>[2x]MEAPEFKDFAKTMVDF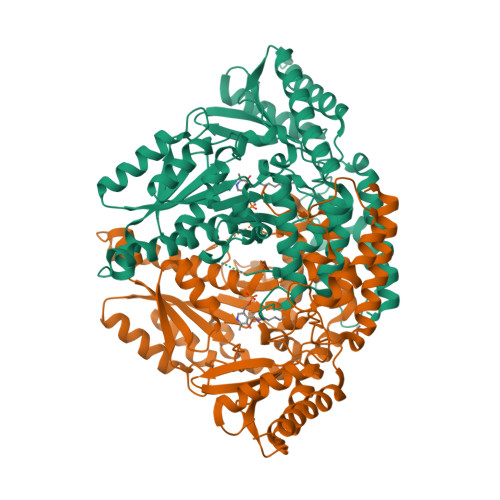IAEYLENIRERRVLPEVKPGYLKPLIPDAAPEKPEKWQDVMQDIERVIMPGVTHWHSPKFHAYFPTANSYPAIVADMLSGAIACIGFTWIASPACTELEVVMMDWLGKMLELPAEFLACSGGKGGGVIQGTASESTLVALLGAKAKKLKEVKELHPEWDEHTILGKLVGYCSDQAHSSVERAGLLGGVKLRSVQSENHRMRGAALEKAIEQDVAEGLIPFYAVVTLGTTNSCAFDYLDECGPVGNKHNLWIHVDAAYAGSAFICPEYRHLMKGIESADSFNFNPHKWMLVNFDCSAMWLKDPSWVVNAFNVDPLYLKHDMQGSAPDYRHWQIPLGRRFRALKLWFVLRLYGVENLQAHIRRHCNFAKQFGDLCVADSRFELAAEINMGLVCFRLKGSNERNEALLKRINGRGHIHLVPAKIKDVYFLRMAICSRFTQSEDMEYSWKEVSAAADEMEQEQ> GNPVTVVTATTGSKQNCTTGEGDYQLVQHEVLCSMKNTYEVLDFLGRGTFGQVVKCWKRGTNEIVAIKILKNHPSYARQGQIEVSILARLSTENADEYNFVRAYECFQHRNHTCLVFEMLEQNLYDFLKQNKFSPLPLKVIRPILQQVATALKKLKSLGLIHADLKPENIMLVDPVRQPYRVKVIDFGSASHVSKTVCSTYLQSRYYRAPEIILGLPFCEAIDMWSLGCVIAELFLGWPLYPGALEYDQIRYISQTQGLPGEQLLNVGTKSTRFFCKETDMSHSGWRLKTLEEHEAETGMKSKEARKYIFNSLDDVAHVNTVMDLEGSDLLAEKADRREFVSLLKKMLLIDADLRITPAETLNHPFVNMKHLLDFPHSNHVKSCFHIMDICKSHLNSCDTNNHN

HIPKs belong to the CMGC group of serine/threonine kinases and are part of the dual-specificity tyrosine phosphorylation-regulated kinase (DYRK) family. DYRKs are named after their characteristic dual-specificity, as they auto-phosphorylate a conserved tyrosine in their activation loop, but phosphorylate substrates on serine and threonine residues. HIPKs are regulators of various signaling pathways and involved in the pathology of cancer, chronic fibrosis, diabetes, and multiple neurodegenerative diseases. Based on a database search, we identified abemaciclib, an FDA-approved Cdk4/Cdk6 inhibitor used for the treatment of metastatic breast cancer, as potent inhibitor of HIPK2, HIPK3, and DYRK1A.

To determine the structure of the human HIPK3 kinase domain, residues 159–562 were expressed in baculovirus infected Sf9 insect cells. Crystals were grown in the presence of ADP and MgCl2 by the hanging drop vapor diffusion method. One HIPK3 monomer forms the asymmetric unit cell of the protein crystal. Despite its presence in the crystallization condition, no crystallographic density was seen for ADP or magnesium, implying that the kinase is in the nucleotide free apo-state. In the structure, a continuous polypeptide chain from residue 184 to 550 was determined for HIPK3, exhibiting the classical kinase fold as seen, e.g., for Cdk219 with an N-terminal lobe (197–278) and a C-terminal lobe (279-526) including a fully ordered activation segment. At the N-terminus, 13 additional residues preceding the canonical kinase domain are seen in the electron density map, forming an extended stretch in an antiparallel conformation to the β1 strand of the N-lobe. Another 24 residues are resolved at the C-terminus extending the chain to position 550 by two helices (αJ and αK) that form an α-barrel with helices αI and αE of the C-lobe at the back of the ATP-binding site. In our crystal structure of HIPK3, the conserved tyrosine Y359 constitutes the only phosphorylated residue. For HIPK3 instead, we find that the phosphate group of pY359 forms a 3.0 Å salt bridge with the side chain of R431, which is part of the HIPK specific insert region. The RYYR motif remains at the same position as in DYRKs and HIPK2, yet, R363 is hydrogen-bonded to the carbonyl group of G401 and R366 forms a tight salt bridge (2.6 Å) to E404. Unexpectedly, the structure of HIPK3 adopts an active conformation with a fully accessible ATP-binding site even though the kinase is in its apo-state.(3S)-3-(2-amino-5-chloro-1H-benzimidazol-1-yl)-N-(cyclohexylmethyl)pentanamide 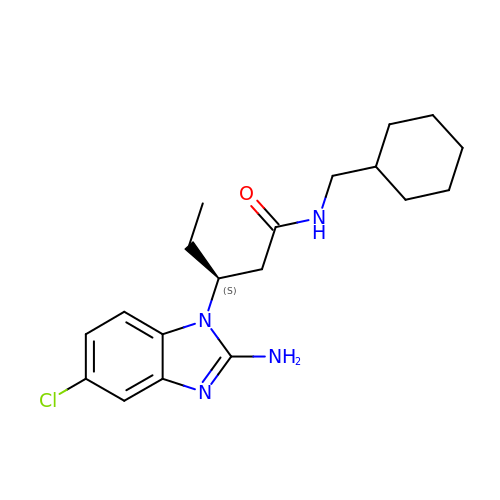| C19 H27 Cl N4 O | UKACQFCXAAAWAE-HNNXBMFYSA-N> MAVVPIRIVGDPVLHTATTPVTVAADGSLPADLAQLIATMYDTM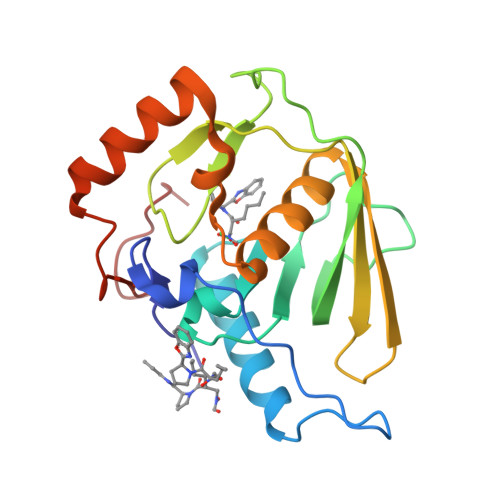DAANGVGLAANQIGCSLRLFVYDCAADRAMTARRRGVVINPVLETSEIPETMPDPDTDDEGCLSVPGESFPTGRAKWARVTGLDADGSPVSIEGTGLFARMLQHETGHLDGFLYLDRLIGRYARNAKRAVKSHGWGVPGLSWLPGEDPDPFGH[[(2~{S})-2-[[6-(4-methylphenyl)thieno[2,3-d]pyrimidin-4-yl]amino]-3-phenyl-propanoyl]amino]phosphonic acid | 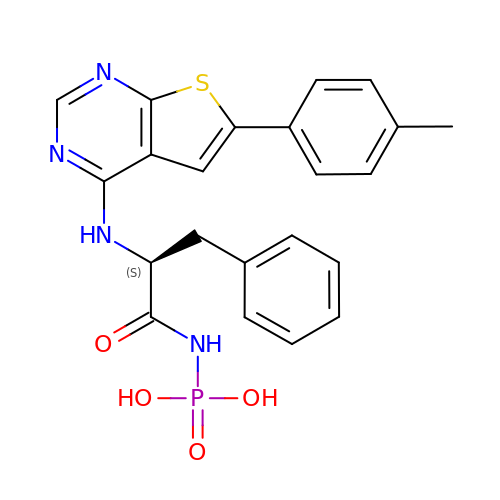C22 H21 N4 O4 P S | FWELKNKHGIBMRD-SFHVURJKSA-N7-oxidanylidene-8-[2-(4-sulfonaphthalen-1-yl)hydrazinyl]-8~{H}-naphthalene-1,3-disulfonic acid | C20 H16 N2 O10 S3 | 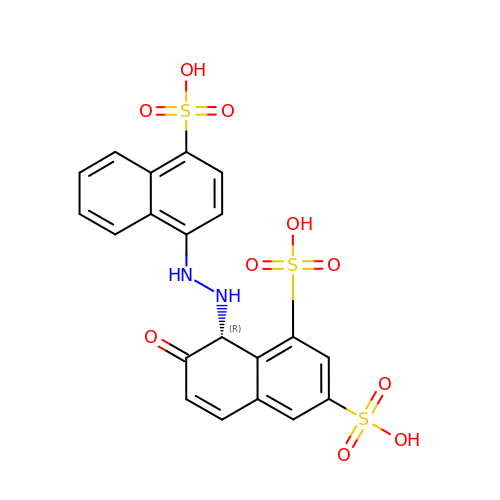DOHFSJYQGWYGDQ-FQEVSTJZSA-N> MPEITRRRALTAAAAVAATASAAVTLAAPAASAAGHHEPAAPESFDEVYKGRRIQGRPAGGGAHHHEHGGGYEVFVDGVQLHVMRNADGSWISVVSQYDPVPTPRAAARAAVDELQGAPLLPFP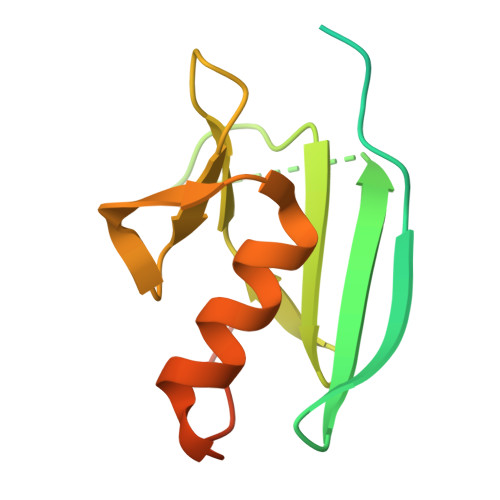ANLEHHHHHH>MTKNPRNNKPKKILDSSYKSKTIWQNYIDALFETFPQLEISEVWAKWDGGNVTKDGGDAKLTANIRTGEHFLKAREAHIVDPNSDIYNTILYPKTGADLPCFGMDLMKF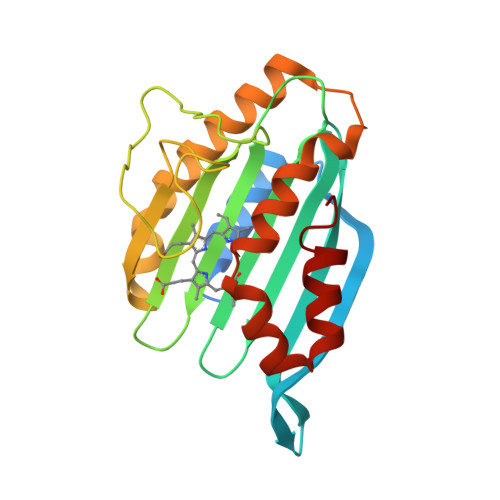SDKKVIIVFDFQHPREKYLFSVDGLPEDDGKYRFFEMGNHFSKNIFVRYCKPDEVDQYLDTFKLYLTKYKEMIDNNKPVGEDTTVYSDFDTYMTELNPVRGYMKNKFGEGRSEAFVNDFLFSYK[2x]>[2x]DFAAKCAGFKTSLKLPNTKVWFTEHVPAGKNITFPDNHPTCTPKSTITDVEICRVAMFVTTGPKSNLTLEAWLPSNWTGRFLSTGNGGMAGCIQYDDVAYGAGFGFATVGANNGHNGTSAVSMYKNSGVVEDYVYRSVHTGTVLGKELTKKFYGKKHTKSYYLGCSTGGRQGWKEAQSFPDDFDGIVAGAPAMRFNGLQSRSGSFWGITGPPGAPTHLSPEEWAMVQKNVLVQC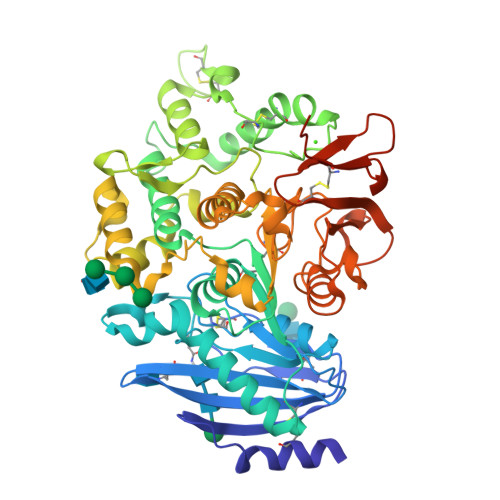DEPLDGVADGILEDPNLCQYRPEALVCSKGQTKNCLTGPQIETVRKVFGPLYGNNGTYIYPRIPPGADQGFGFAIGEQPFPYSTEWFQYVIWNDTKWDPNTIGPNDYQKASEVNPFNVETWEGDLSKFRKRGSKIIHWHGLEDGLISSDNSMEYYNHVSATMGLSNTELDEFYRYFRVSGCGHCSGGIGANRIGNNRANLGGKEAKNNVLLALVKWVEEGQAPETITGVRYVNGATTGKVEVERRHCRYPYRNVWDRKGNYKNPDSWKCELPLEQKLISEEDLNSAVDHHHHHH>[6x]MSEITGLFKDLTKVKHARNGRLASWDQRGKNQDYWEIPAGESITLGEIEGPGCITHM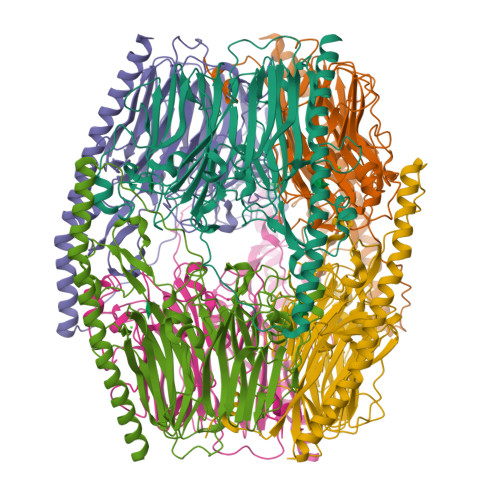WMTSSCRKVVAPSILDPELNASAAPVMEIHPALGVIWDAYDPFYYRKALIKITWDDQDTPSVLVPFGDFFCIGNSYPGNFSSLPFNVSLKPEEAGKFGAPCSVSCYFPMPFNKKAKIEIVNDNELPFILYFNIDYEMYGEPLPEDTAYFHAAWHRENPCNGWGPELQVNSPEVNNVTNFKGENNYTVLDVEGTGHYVGCNLTVKHFQGSWWGEGNDMFFIDGEEYPSLNGTGTEDYFNHAWGMQRNAYPFFGTIVHEGDTDGFQVSYRWHITDPVRFEKHLKVTIEHGHANQLSDDWSSTAYWYQILPTASRITIAPVEDRLPVVPQLPERKLVLPQLTEEQQAARDTYQKRWKDYEPRRDTQFRIKEDKARRESKLNTEFAKKLRDAFDAEREQLEHHHHHH> GSLYRQRYQFVKNLVDQHEPKKVADLGCGDTSLLRLLKVNPCIELLVGVDINEDKLRWRGDSLAPFLGDFLKPRDLNLTITLYHGSVVERDSRLLGFD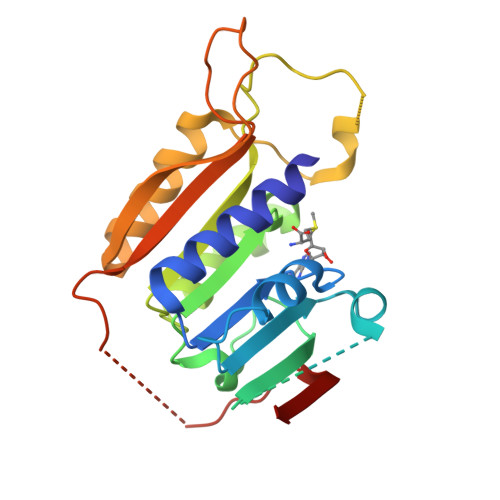LITCIELIEHLDSGDLARFPEVVFGYLSPSMIVISTPNSEFNPLFPSVTLRDSDHKFEWTRMEFQTWALYVANRYDYSVEFTGVGEPPAGAENVGYCTQIGIFRKNGGKATESCLSEQHDQHVYKAVFTTSY> MHSTNNNSNKRNNEEKHKQPEIDSSANNGEGTSGTRAQTVGDTATEAGVRNETEAGASTRRQTDGTGLSGTNAKIATASSARQADVEKPADVTFTIENVDDVGIMQQKKPPTVVQSRTDVFNEQFANEALHPTTKVIFNGLDVNTEVQPLSDDFKQISDPKGYLTYSVKYEDQFTKKDKLRASEADDRIVGPTVNLFKYGAAVVNIDLNRDFFDTATGIDLTKGIPLVQDLLVPIGVTAGAEQSAEYVSGLLMVLFKVMTDNRLVIVGETTTPMSNTLSTVVNNVLRTTYHNNVGVNPALLRDFTQVNWLNRDITNMLQQAGTKYGLGLTETRLDYVRLVKTIVGHALNIDHFAASVLNINLRALMEANVTADDRIKALQAHSMISTQFHGPNQGALRPELAFDHDHIIRCLMLAAANYPRLEGIIVQINTGYVASANVIRPVSEKRYFPENLEQNQSAARLVSAVKARASEADISSIHLAIAREVSPMFNVHELKKIAESFEDPSSIVVVLEFILFALFFPTEFNRIKGDIQNVLLLFFSRWYPVEYGIFVQRGATYTINAAGEFEFSGRNEKWDQALYLSEHFPALFSDVPLAGANTIIAIMRLFTPQGFLRTDDLAIAANFPRASRNPQTYIPYTNQRGTVTNEFASRFRTIVATLANVVNERAVQDDMQKATRSCTKQWLRHLETQFDNIAVAHTDHLSVVYATMSNFMLNFTNNFSGNHATFKPDQYVITSPEGSYKPIIERQGETVDGLTIIDTSIVWPILCQCTYPLVRQSGKGVDAVSIMEEIVYPDPSTTLSQSLSVAQVLSKLTLPDAFINMILSGGDSVVMRTYQTEADDDLDEGIRM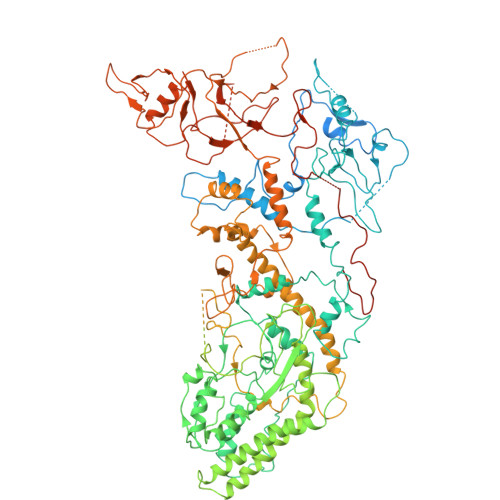TTYDQYLSHIRERLHITNVPDPIYITGASTPDQIAASVQATHVAVVLYQSGVINGPASTYLRENEVLVVMPDYYDVVSRFANANLQMNNNRYHESVLEIADIFDQADFIQTSDAVRQLRALMPTLSTSQIRHAIERIAQITDVDSTDYGKLTLRFLGTLTRSLKMQNAQIRRIRPDGTVLRYDDQIDIEAFRWSRYFLDELQLRRLSVGLRLITNPRIARRFNGVRIMYLTDDDPDPDFVPDVPEGYVAVQYAHRLFSSSLANKRNRVTYTHPPTGMAYPSPTGRPHVHMTINERAGMSKLVADNIIASVIKSNWVVDILDIEYTAEVMTPSEGYTQHVDAESIMTAPKGKLFHLQFMDGLLRPEPSAFDPPASGEDMRLIYPLQPISVARSMRAIVNHNEVDRPRGAVAPSSYEMDTGTLSRNGDLLYSPVANGQVGIPKLEVDHISFSNVVSMMTANIRTGDDMAVERVNPDDVRAINIRNA> HYQETQAVEAGEKTVEQFVQALNKGDYNKAAEMTSKKAANKSALSEKEILDKYQNIYGAADVKGLQISNLKVDKKDDSTYSFSYKAKMNTSLGELKDLSYKGTLD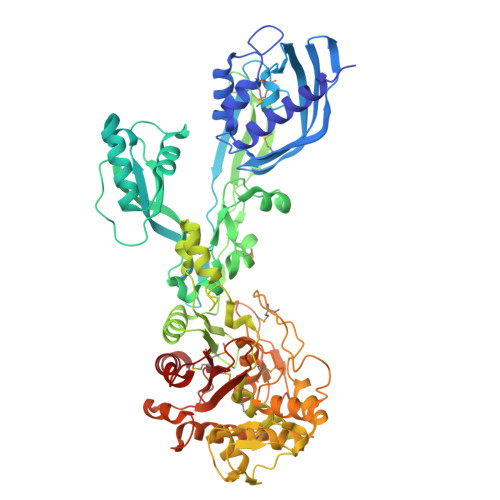RNDGQTTINWQPNLVFPEMEGNDKVSLTTQEAARGNIIDRNGEPLATTGKLKQLGVVPSKLGDGGEKTANIKAIASSFDLTEDAINQAISQSWVQPDYFVPLKIIDGATPELPAGATIQEVDGRYYPLGEAAAQLIGYVGDITAEDIDKNPELSSNGKIGRSGLEMAFDKDLRGTTGGKLSITDADGVEKKVLIEHEVQNGKDIKLTIDAKAQKTAFDSLGGKAGSTVATTPKTGDLLALASSPSYDPNKMTNGISQEDYKAYEENPEQPFISRFATGYAPGSTFKMITAAIGLDNGTIDPNEVLTINGLKWQKDSSWGSYQVTRVSDVSQVDLKTALIYSDNIYMAQETLKMGEKKFRTGLDKFIFGEDLDLPISMNPAQISNEDSFNSDILLADTGYGQGELLINPIQQAAMYSVFANNGTLVYPKLIADKETKDKKNVIGETAVQTIVPDLREVVQDVNGTAHSLSALGIPLAAKTGTAEIKEKQDEKGKENSFLFAFNPDNQGYMMVSMLENKEDDDSATKRASELLQYLNQNYQ>MAYRICLIEGDGIGYEVIPAARRVLEATGLPLEFVEAEAGWETFERRGTSVPEETVVKILSCHATLFGAATIPTRKVPGFFGAIMALRRRLDLYANVRPAKSRPVPGSRPGVDLVIVRENTEGLYVEQERRYLDVAIADAVISKKASERIGRAALRIAEGRPRKTLHIAHKANVLPLTQGLFLDTVKEVAKDFPLVNVQDIIVDNCATQLVMRPERYDVIVTTNLLGDILSDL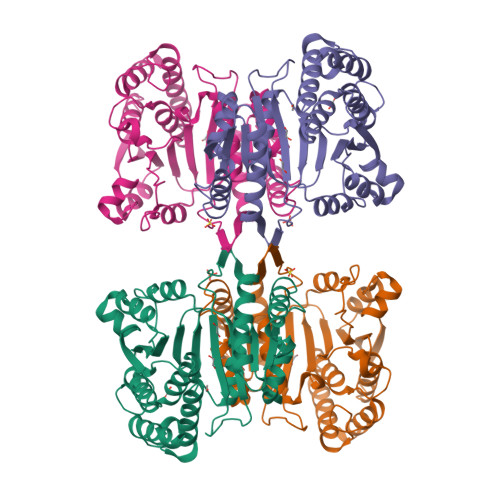AAGLMGGLGLAPSGNIGDTTAVFEPVHGSAPDIAGKGIANPTAAILSAAMMLDYLGEKEAAKRVEKAVDLVLERGPMTPDLGGDATTEAFTEAVVEALKSL[4x]> TTHFSIVDKDGNAVSNTYTLNWDFGSGVVVKGAGFLLNDEMDDFSSKPGVANAFGVVGSDANAIEPGKRMLSSMSPSIVTRDGHVSLVLGTPGGSRIFTSIFQVLNNVYDFHLPLEKAVAAQRVHHQLLPKDTIYYD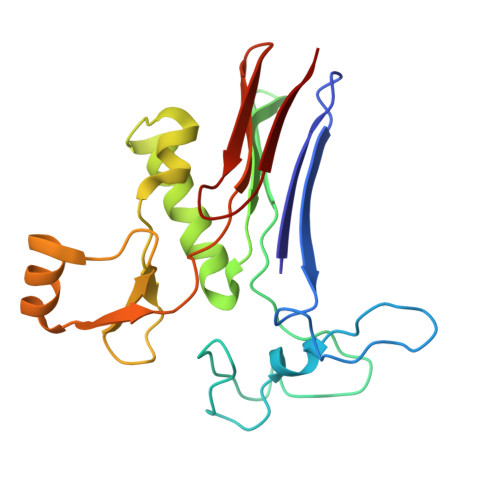AYAPLTGKVADELKAMGYTLEDQGWNMGDIQAIRVNGKALETASDPRGRGVGMVVKP>GSCPKNWKSFSSNCYFISTESASWQDSEKDCARMEAHLLVINTQEEQDFIFQNLQEESAYFVGLSDPEGQRHWQWVDQTPYNESSTFWHPREPSDPNERCVVLNFRKSPKRWGWNDVNCLGPQRSVCEMMKI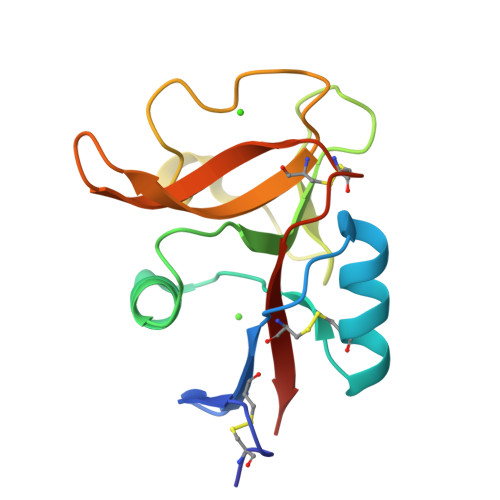HL[4x]> MGMAYSYTEKKRIRKDFSKLPDVMDVPYLLAIQLDSYREFLQAGATKEQFRDVGLHAAFKSVFPIISYSGNAALEYVGYRLGEPAFDVKECVLRGVTFAVPLRVKVRLIIFDRESSNKAIKDIKEQEVYMGEIPLMTENGTFIINGTERVIVSQLHRSPGVFFDHDRGKTHSSGKLLYSARIIPYRGSWLDFEFDPKDCVFVRIDRRRKLPASVLLRALGYSTEEILNAFYATNVFHIKGETLNLELVPQRLRGEVASIDIKDGSGKVIVEQGRRITARHINQLEKAGVSQLEVPFDYLIGRTIAKAIVHPATGEIIAECNTELTLDLLAKVAKAQVVRIETLYTNDIDCGPFISDTLKIDNTSNQLEALVEIYRMMRPGEPPTKEAAETLFGNLFFSAERYDLSAVGRMKFNRRIGRTEIEGPGVLSKEDIIDVLKTLVDIRNGKGIVDDIDHLGNRRVRCVGEMAENQFRVGLVRVERAVKERLSMAESEGLMPQDLINAKPVAAAIKEFFGSSQLSQFMDQNNPLSEITHKRRVSALGPGGLTRERAGFEVRDVHPTHYGRVCPIETPEGPNIGLINSLATYARTNKYGFLESPYRVVKDSLVTDEIVFLSAIEEADHVIAQASATLNEKGQLVDELVAVRHL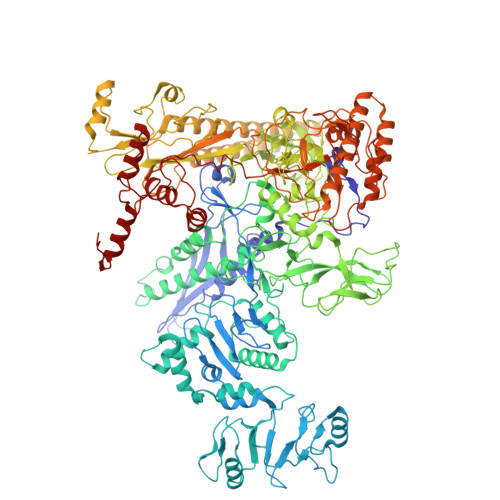NEFTVKAPEDVTLMDVSPKQVVSVAASLIPFLEHDDANRALMGSNMQRQAVPTLRADKPLVGTGMERNVARDSGVCVVARRGGVIDSVDASRVVVRVADDEVETGEAGVDIYNLTKYTRSNQNTCINQRPLVSKGDVVARGDILADGPSTDMGELALGQNMRVAFMPWNGFNFEDSICLSERVVQEDRFTTIHIQELTCVARDTKLGPEEITADIPNVGEAALNKLDEAGIVYVGAEVQAGDILVGKVTPKGETQLTPEEKLLRAIFGEKASDVKDTSLRVPTGTKGTVIDVQVFTRDGVERDSRALSIEKMQLDQIRKDLNEEFRIVEGATFERLRAALVGAKAEGGPALKKGTEITDDYLDGLERGQWFKLRMADDALNEQLEKAQAYISDRRQLLDDKFEDKKRKLQQGDDLAPGVLKIVKVYLAIKRRIQPGDKMAGRHGNKGVVSVIMPVEDMPHDANGTPVDIVLNPLGVPSRMNVGQILETHLGLAAKGLGEKINRMLEEQRKVAELRKFLHEIYNEIGGREENLDELGDNEILALAKNLRGGVPMATPVFDGAKEREIKAMLKLADLPESGQMRLFDGRTGNQFERPTTVGYMYMLKLNHLVDDKMHARSTGSYSLVTQQPLGGKAQFGGQRFGEMEVWALEAYGAAYTLQEMLTVKSDDVNGRTKMYKNIVDGDHRMEAGMPESFNVLIKEIRSLGIDIELETE>[2x]MTINYHELETSHGRIAVRESEGEGAPLLMIHGNSSSGAIFAPQLEGEIGKKWRVIAPDLPGHG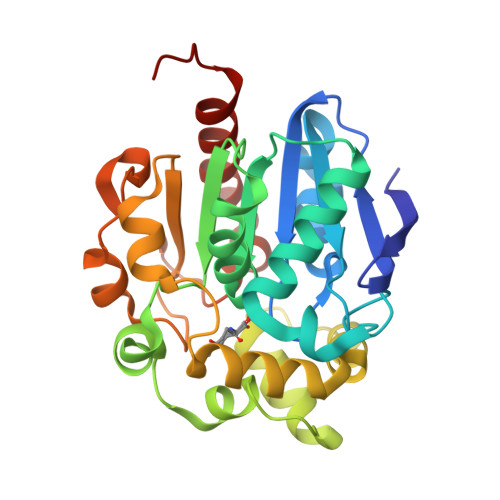KSTDAIDPDRSYSMEGYADAMTEVMQQLGIADAVVFGWSLGGHIGIEMIARYPEMRGLMITGTPPVAREEVGQGFKSGPDMALAGQEIFSERDVESYARSTCGEPFEASLLDIVARTDGRARRIMFEKFGSGTGGNQRDIVAEAQLPIAVVNGRDGPFVELDFVSKVKFGNLWEGKTHVIDNAGHAPFREAPAEFDAYLARFIRDCTQLEHHHHHH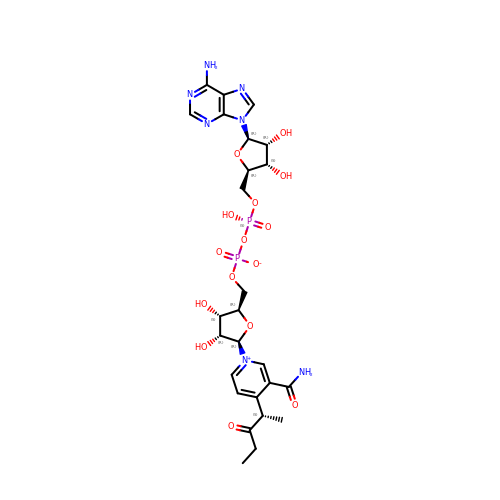NICOTINAMIDE ADENINE DINUCLEOTIDE 3-PENTANONE ADDUCT | C26 H35 N7 O15 P2 | BZJFKYRGSZWSLT-YLIVDTKOSA-N N-(8-methyl-1,2,3,4-tetrahydroquinolin-5-yl)acetamide | C12 H16 N2 O | 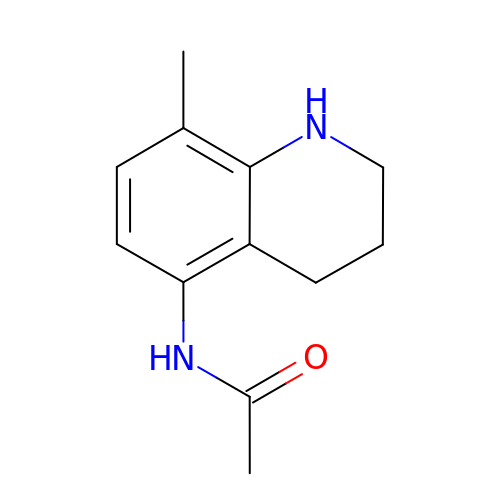RYRDUZSMONMBBE-UHFFFAOYSA-N Nylon hydrolase (NylC) is one of the three enzymes responsible for the endo-type degradation of the by-products of nylon-6 manufacture (cyclic and linear oligomers of 6-aminohexanoate (Ahx) with a degree of polymerization greater than three) and various aliphatic nylons (e.g., nylon-6 and nylon-66). However, the post-translational autocleavage of the nascent polypeptide between Asn266 and Thr267 generates an active enzyme with an α subunit (27 kDa) and a β subunit (9 kDa). Based on the X-ray-crystallographic structure of NylCA, we reported that four αβ heterodimers (molecules A-D) form a doughnut-shaped quaternary structure. In addition, we proposed that the nucleophilic N-terminal residue Thr267 in the β subunit functions as a catalytic residue for either autocleavage (from precursor to active enzyme) or substrate hydrolysis.

To extensively analyze the effect of amino acid substitution at position 122, we constructed 10 new mutants in which Asp122 of NylCp2 was replaced with other amino acids by site-directed mutagenesis. The values of Tm (melting point of the heat denaturation) and ΔH (change in enthalpy for the global unfolding of proteins) were determined by regression analysis using nonlinear least-squares fitting of the CD melting curve. The Tm values increased in the order of Asp122 (wild-type NylCp2) < Leu < Gln < Asn < Arg < Lys < Val < Gly and ranged from 52.9 °C to 75.1 °C (type 1 mutation in Fig. 2). However, the D2 symmetry was partly altered by mutations at position 122. Plotting the protein stability (Tm value) estimated from the CD analyses against the distance between the two monomer molecules revealed that the protein stability exhibited an inverse correlation with the a2/a1 ratio (index of symmetry). In other words, the ratio changed from 0.979 to 1.197 from the wild-type (Asp122) to the mutant (Arg122, Lys122, Val122, and Gly122) enzyme, although this value should be equal to one for a perfectly symmetric structure. A clearer correlation was found between thermostability and the nearest distance between the side-chain atoms on helix α2 and helix α1. Notably, this distance decreased with an almost linear correlation with increasing thermostability in the wild-type and mutant enzymes. The side-chain atoms of Lys122 existed as two conformers, with the distance of one conformer showing a linear relationship with thermostability.

>MNTTPVHALTDIDGGIAVDPAPRLAGPPVFGGPGNDAFDLAPVRSTGREMLRFDFPGVSIGAAHYEEGPTGATVIHIPAGARTAVDARGGAVGLSGGYDFNHAICLAGGAGYGLEAGAGVSKALLERLEHRTGFAELQLVSSAVIYDFSARSTAVYPDKALGRAALEFAVPGEFPQGRAGAGMSASAGKVDWDRTEITGQGAAFRRLGDVRILAVVVPNPVGVIVDRAGTVVRGNYDAQTGVRRHPVFDYQEAFAEQVPPVTEAGNTTISAIVTNVRMSPVELNQFAKQVHSSMHRGIQPFHTDMDGDTLFAVTTDEIDLPTTPGSSRGRLSVNATALGAIASEVMWDAVLEAGK[2x]>SNAMATLTEDDVLEQLDAQDNLFSFMKTAHSILLQGIRQFLPSLFVDNDEEIVEYAVKPLLAQSGPLDDIDVALRLIYALGKMDKWLYADITHFSQYWHYLNEQDETPGFADDITWDFISNVNSITRNATLYDALKAMKFADFAV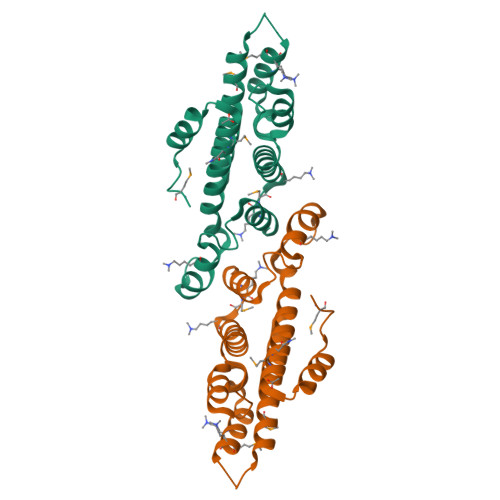WSEARFSGMVKTALTLAVTTTLKELTP[4x]At the core of HSV-1 replication initiation is the OBP, a 94 kDa protein encoded by the UL9 gene. As an essential component of the viral replication machinery, OBP integrates multiple critical functions: origin recognition, DNA binding, and ATP-dependent helicase activity. OBP consists of two major functional domains: an N-terminal helicase-like domain (residues 1–535) and a C-terminal origin-binding domain (residues 536–851). The structures reveal a head-to-tail dimer architecture, with DNA binding on one side.

The second structure captures OBP bound to the complete OriS recognition site, in complex with a non-hydrolyzable ATP analog (ATPγS). In our OBP + OriS + ATPγS complex, we observe both the ATP analog and a coordinated Mg2+ ion, capturing the nucleotide-bound state. ATPγS binding induces subtle closure of the pocket's lower half and a shift of the motif I P-loop, suggesting conformational changes that may couple ATP hydrolysis to DNA unwinding. Within this pocket, we observe a seemingly unusual nucleotide interaction pattern: K87 of motif I contacts the α- and β-phosphates of ATPγS, while backbone amides from S85, G86, K87, and T88 form hydrogen bonds with the α-phosphate. This arrangement differs from other helicases, where the equivalent conserved lysine typically contacts the β- and γ-phosphates. Therefore, our structure potentially represents a non-catalytic state before ATP adopts a position in its pocket that is consistent with turnover. Within motif Ia, our structure shows that R112 reorients to interact with the γ-phosphate of ATPγS. Motif VI exhibits an unexpected arrangement where R389 directly contacts the γ-phosphate of ATPγS, while R387, despite its conservation, remains too distant for ATP interaction. The catalytic Mg2+ ion is coordinated by D174 and E175 within motif II, underscoring their critical role in helicase activity, as evidenced by the loss of function in E175A mutants. Each monomer threads its C-terminal end through its partner molecule, bringing it into close proximity with the ATP-binding pocket in the other monomer.

>[2x]MWSHPQFEKSAMPFVGGAESGDPLGAGRPIGDDECEQYTSSVSLARMLYGGDLAEWVPRVHPKTTIERQQHGPVTFPNASAPTARCVTVVRAPMGSGKTTALIRWLREAIHSPDTSVLVVSCRRSFTQTLATRFAESGLVDFVTYFSSTNYIMNDRPFHRLIVQVESLHRVGPNLLNNYDVLVLDEVMSTLGQLYSPTMQQLGRVDALMLRLLRTCPRIIAMDATANAQLVDFLCGLRGEKNVHVVVGEYAMPGFSARRCLFLPRLGTELLQAALRPPGPPSGPSPDASPDARGATFFGELEARLGGGDNICIFSSTVSFAEIVARFCRQFTDRVLLLHSLTPLGDVTTWGQYRVVIYTTVVTVGLSFDPLHFDGMFAYVKPMNYGPDMVSVYQSLGRVRTLRKGELLIYMDGSGARSEPVFTPMLLNHVVSSCGQWPAQFSQVTNLLCRRFKGRCDASACDTSLGRGSRIYNKFRYKHYFERCTLACLSDSLNILHMLLTLNCIRVRFWGHDDTLTPKDFCLFLRGVHFDALRAQRDLRELRCRDPEASLPAQAAETEEVGLFVEKYLRSDVAPAEIVALMRNLNSLMGRTRFIYLALLEACLRVPMATRSSAIFRRIYDHYATGVIPTINVTGELELVALPPTLNVTPVWELLCLCSTMAARLHWDSAAGGSGRTFGPDDVLDLLTPHYDRYMQLVFELGHCNVTDGLLLSEEAVKRVADALSGCPPRGSVSETDHAVALFKIIWGELFGVQMAKSTQTFPGAGRVKNLTKQTIVGLLDAHHIDHSACRTHRQLYALLMAHKREFAGARFKLRVPAWGRCLRTHSSSANPNADIILEAALSELPTEAWPMMQ> PPKRLTREAMRNYLKERGDQTVLILHAKVAQKSYGNEKRFFCPPPCVYLMGSGWKKKKEQMERDGCSEQESQPCAFIGIGNSDQEMQQLNLEGKNYCTAKTLYISDSDKRKHFMLSVKMFYGNSDDIGVFLSKRIKVISKPSKKKQSLKNADLCIASGTKVALFNRLRSQTVSTRYLHVEGGNFHASSQQWGAFYIHLLDDDESEGEEFTVRDGYIHYGQTVKLVCSVTGMALPRLIIRKVDKQTALLDADDPVSQLHKCAFYLKDTER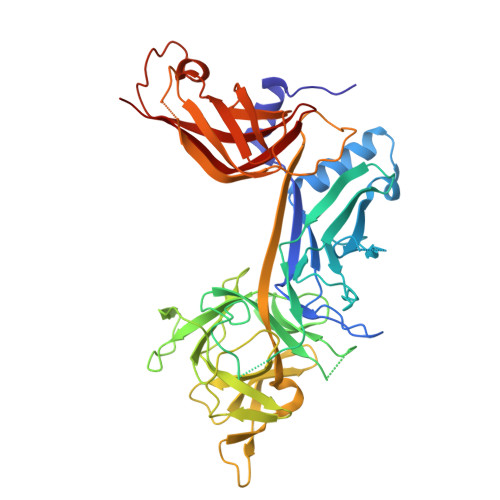MYLCLSQERIIQFQATPCPKEQNKEMINDGASWTIISTDKAEYTFYEGMGPVLAPVTPVPVVESLQLNGGGDVAMLELTGQNFTPNLRVWFGDVEAETMYRCGESMLCVVPDISAFREGWRWVRQPVQVPVTLVRNDGVIYSTSLTFTYTPEP>[2x]SGFVCNTCPEKWINFQRKCYYFGKGTKQWVHARYACDDMEGQLVSIHSPEEQDFLTKHASHTGSWIGL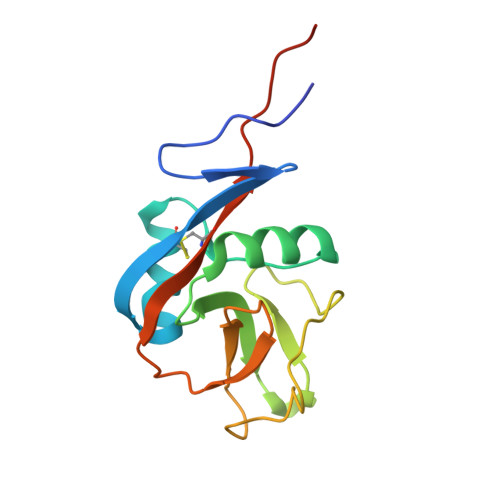RNLDLKGEFIWVDGSHVDYSNWAPGEPTSRSQGEDCVMMRGSGRWNDAFCDRKLGAWVCDRLATCTPPASEGSAE Ureases are nickel-metalloenzymes produced in plants, fungi, and bacteria, but not in animals. They facilitate nitrogen fixation by metabolizing urea, but in some pathogenic bacteria they serve a dual function and consume ammonia to promote survival in acidic environments. Y. enterocolitica urease comprises three polypeptide chains (ureA, ureB, and ureC), an architecture similar to that of K. aerogenes urease and has been biochemically characterized previously. The active site contains two Ni2+ ions which are coordinated by six different amino acids.

We have determined the structure of a dodecameric urease assembly, a metalloenzyme from the pathogen Y. enterocolitica at an overall resolution of 1.98 Å using cryo-EM. The structure shows that Y. enterocolitica urease assembles into a dodecameric hollow sphere with a [[αβγ]3]4 oligomeric assembly structure of tetrahedral symmetry. The homo-trimer is arranged in a tetramer-of-trimers making the full complex a dodecamer of the hetero-trimer. There are four large oval shaped holes between the trimers (64 Å long, 12 Å wide, high electrostatic potential) and four smaller holes at the center of the trimer with a diameter of 6 Å (low electrostatic potential), as shown in Fig. 2b, and the center of the enzyme assembly is hollow. A tightly embedded kinked loop is interacting with neighboring domains and is potentially responsible for the assembly of the oligomer. Furthermore, the high resolution allows for a detailed description of the nickel-metallo-center and the active site. The active site is located on the ureC protein at the edge of the hetero-trimer and is wedged in between the ureA and ureB proteins of the next hetero-trimer in the homo-trimeric assembly. Ni(1) is additionally coordinated by His224, His251 and His277 and Ni(2) by His139, His141, and Asp365. The mobile flap of the cryo-EM structure presented here is modeled in an open position, however the local resolution is lower than in the surrounding areas, indicating flexibility. The distance between the Ni2+ ions is 3.7 Å in X-ray structures of K. aerogenes and S. pasteurii, but only 3.2 Å in the Y. enterocolitica cryo-EM model. Finally, we noticed that radiation damage can partially explain the shorter distance observed between the nickel atoms in the active site, possibly by a stronger ferromagnetic interaction after deprotonation of the bridging hydroxide molecule.

>SEQNTPLGGCILADTPITFNENKPVTKVKVRNTGDRPIQVGSHFHFFEVNRALEFDRAAAYGKRLNISSTTAIRFEPGDETEVPLIPFGGKQTLYGFNNLVDGWTGEGVVPNSERPDKLEAIRRAAERGFKS[12x];>PQISRQEYAGLFGPTTGDKIRLGDTNLFIEIEKDLRGYGEESVYGGGKSLRDGMGANNHLTRDNGVLDLVITNVTIVDARLGVIKADVGIRDGKIAGIGKSGNPGVMDGVTPGLVVGVSTDAISGEHLILTAAGIDTHIHLISPQQAYHALSNGVATFFGGGIGPTDGTNGTTVTPGPWNIRQMLRSVEGLPVNVGILGKGNSYGRGPLLEQAIAGVVGYKVHEDWGATANALRHSLRMADEMDIQVSVHTDSLNECGYVEDTIDAFEGRTIHTFHTEGAGGGHAPDIIRVASQPNVLPSSTNPTLPYGVNSQAELFDMIMVCHNLNPNVPADVSFAESRVRPETIAAENVLHDMGVISMFSSDSQAMGRVGENWLRVMQTANAMKASRGKLPEDAPGNDNFRVLRYVAKITINPAIAQGVSHVIGSVEVGKMADLVLWDPRFFGAKPKMVIKGGMINWAAMGDPNASLPTPQPVFYRPMFGAMGKTMQDTCVTFVSQAALDDGVKEKAGLDRQVIAVKNCRTISKHDLVRNDQTPNIEVDPETFAVKVDGVHATCEPIDTAAMNQRYFFG[12x];>[12x]MQLTPREVEKLMIYTLSDVAFKRKARGLKLNYPEAVSIITVTAMEGARDGKSVEDVMKEASKVLTKDDVMDGVADLIPNVQVEAIFTDGSRLVTVHDPIK> MAGIAMKLAKDREAAEGLGSHERAIKYLNQDYETLRNECLEAGALFQDPSFPALPSSLGFKELGPYSSKTRGIEWKRPTEICADPQFIIGGATRTDICQGALGDSWLLAAIASLTLNEEILARVVPLDQSFQENYAGIFHFQFWQYGEWVEVVVDDRLPTKDGELLFVHSAEGSEFWSALLEKAYAKINGCYEALSGGATTEGFEDFTGGIAEWYELRKPPPNLFKIIQKALEKGSLLGCSIDITSAADSEAVTYQKLVKGHAYSVTGAEEVESSGSLQKLIRIRNPWGQVEWTGKWNDNCPSWNTVDPEVRANLTERQEDGEFWMSFSDFLRHYSRLEICNLTPDTLTCDSY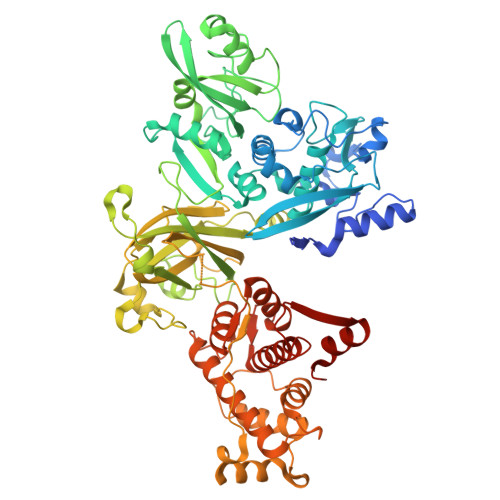KKWKLTKMDGNWRRGSTAGGCRNYPNTFWMNPQYLIKLEEEDEDDEDGERGCTFLVGLIQKHRRRQRKMGEDMHTIGFGIYEVPEELTGQTNIHLSKNFFLTTRARERSDTFINLREVLNRFKLPPGEYVLVPSTFEPHKNGDFCIRVFSEKKADYQTVDDEIEANIEEIEANEEDIGDGFRRLFAQLAGEDAEISAFELQTILRRVLAKREDIKSDGFSIETCKIMVDMLDEDGSGKLGLKEFYILWTKIQKYQKIYREIDVDRSGTMNSYEMRKALEEAGFKLPCQLHQVIVARFADDELIIDFDNFVRCLVRLEILFKIFKQLDPENTGTIQLDLISWLSFSVLGKLAAALEHHHHHH>[2x]MKFGKNLPRNQVPEWAGSYINYKGLKKLVKAAAESAKDGQPVDLAEFFFALDRNLEDVDSFYNKKFADACRRLKVLQDRYGTTPEVVVNLDDDEAEE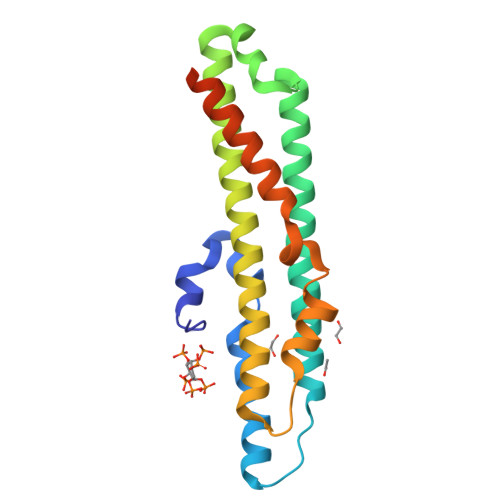LMGALLELRSQLRKLQWFGEINRRGFIKITKKLDKKVPNTTTQHRYISTKVDPKPFAKDTTVARILTEINRWISVLGDARNVEDNRSLEHHHHHH>SNAVEGIPQPEFDRGFLRPFGAKMKFLKPDQVQKLSTDDLITYMAEKDKNVRDLAIKLRDAKQDSTKNGTPEIKQTYDKAYEKTKAAAEKLVSEESLTRDALLKLTEEQYVEKAALFDKDVYRNNLKRQTYEKLLRSETDVL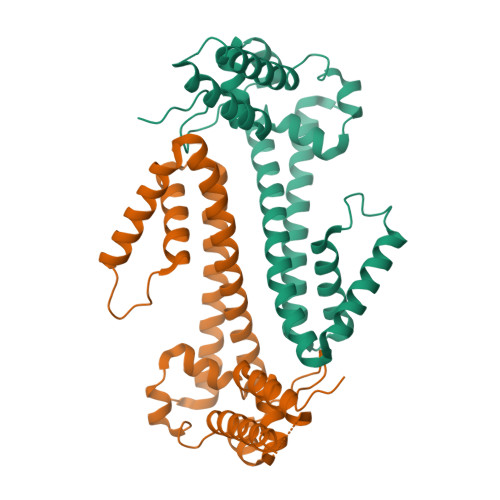YREVARIFIAREGEPALTAKIERLALTLENNADTRSKPIDYLAIAADFLKNQANLHADDPELNLYKAEIKAREIEANRAMKEALKGADKLFKRNKILKSPDM[8x]> SNAMLRYGDTEICIDPSESVLHLLGKKYTMLIISVLGNGSTRQNFNDIRSSIPGISSTI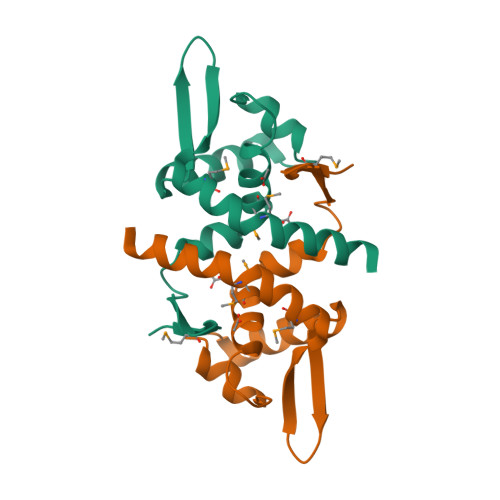LSRRIKDLIDSGLVERRSGQITTYALTEKGMNVRNSLMPLLQYISVLDRNGD> MAFPAGFGWAAATAAYQVEGGWDADGKGPCVWDTFTHQGGERVFKNQTG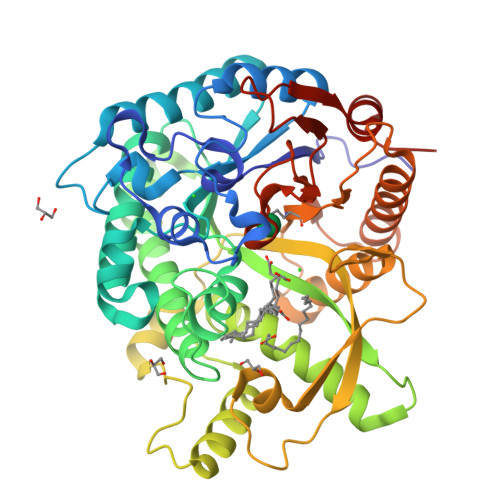DVACGSYTLWEEDLKCIKQLGLTHYRFSLSWSRLLPDGTTGFINQKGIDYYNKIIDDLLKNGVTPIVTLYHFDLPQTLEDQGGWLSEAIIESFDKYAQFCFSTFGDRVKQWITINQANVLSVMSYDLGMFPPGIPHFGTGGYQAAHNLIKAHARSWHSYDSLFRKKQKGMVSLSLFAVWLEPADPNSVSDQEAAKRAITFHLDLFAKPIFIDGDYPEVVKSQIASMSQKQGYPSSRLPEFTEEEKKMIKGTADFFAVQYYTTRLIKYQENKKGELGILQDAEIEFFPDPSWKNVDWIYVVPWGVCKLLKYIKDTYNNPVIYITENGFPQSDPAPLDDTQRWEYFRQTFQELFKAIQLDKVNLQVYCAWSLLDNFEWNQGYSSRFGLFHVDFEDPARPRVPYTSAKEYAKIIRNNGLEAHL> MTWLTKIVPDLRYRQTRADFRTAGNLHRKLIRLSSDLGEERIANPRQQSGLLFRIEETRNELYLLVQSHSPLRVDRLGPGYHGVQMRNLDPFLARLDKGSRVRYRIVASPT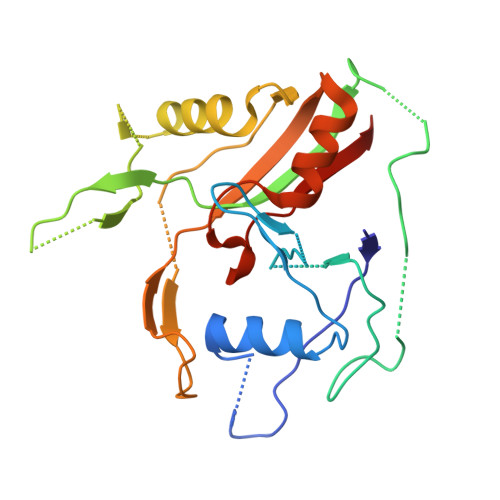KRLGRSENNTQRLGLKEPPKKPREYTWALRGAAAEEWWHSRAAANGLELLSTYAQTLDDVRDPGTADRSRKIRHPAVRFDGEAVISDVDAVRHAVLNGIGRGKSYGCGLLSLALIEEGEHG>[4x]SNAGFVVKVRGLPWSCSADEVQRFFSDCKIQNGAQGIRFIYTREGRPSGEAFVELE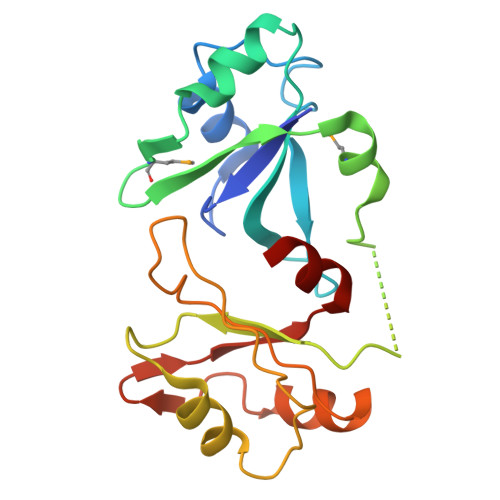SEDEVKLALKKDRETMGHRYVEVFKSNNVEMDWVLKHTGPNSPDTANDGFVRLRGLPFGCSKEEIVQFFSGLEIVPNGITLPVDFQGRSTGEAFVQFASQEIAEKALKKHKERIGHRYIEIFKSSRAEVRTH>[2x]PEERQISVLSINQSLDYLLEKGASVVRFGDGEMDLVAGRSIVYQDFDPELSARLREIMSMESDERLMVCLPDVFTGLERYSIDAQNFWSLNHLPHFLEKYKNICRAPWYGSTFISRPYIDLEDKTPSVGYFAK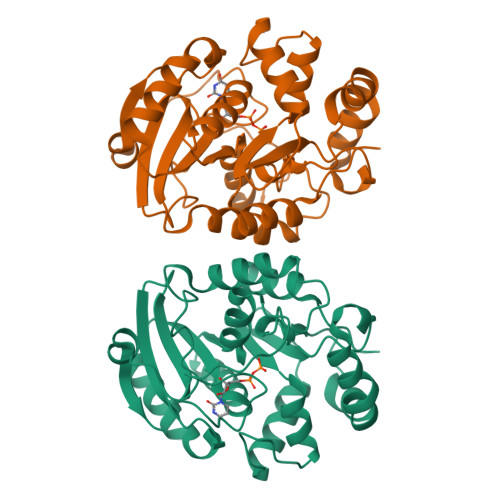LKQLWQDKDLLIVEGLTSRSGVGNDLFDGARSIKRIICPSRNAYSKLEAIKQAVREHADNRLILTMLGPTAKVLVYDLVQEGYRALDIGHIDSEYEWFQMGASHKVKLSHKHTAEHNFDQDIEFRDDQAYDSQIVANLAQE>MSTYEGRWKTVKVEIEDGIAFVILNRPEKRNAMSPTLNREMIDVLETLEQDPAAGVLVLTGAGEAWTAGMDLKEYFREVDAGPEILQEKIRREASQWQWKLLRMYAKPTIAMVNGWCFGGGFSPLVACDLAICADEATFGLSEINWGIPPGNLVSKAMADTVGHRQSLYYIMTGKTFGGQKAAEMGLVNESVPLAQLREVTIELARNLLEKNPVVLRAAKHGFKRCRELTWEQNEDYLYAKLDQSRLLDTEGGREQGMKQFLDDKSIKPGLQAYKR[4x];> MSTYEGRWKTVKVEIEDGIAFVILNRPEKRNAMSPTLNREMIDVLETLEQDPAAGVLVLTGAGEAWTAGMDLKEYFREVDAGPEILQEKIRREASQWQWKLLRMYAKPTIAMVNGWCFGGGFSPLVACDLAICADEATFGLSEINYGIPPGNLVSKAMADTVGHRQSLYYIMTGKTFGGQKAAEMGLVNESVPLAQLREVTIELARNLLEKNPVVLRAAKHGFKRCRELTWEQNEDYLYAKLDQSRLLDTEGGREQGMKQFLDDKSIKPGLQAYKR;> MSTYEGRWKTVK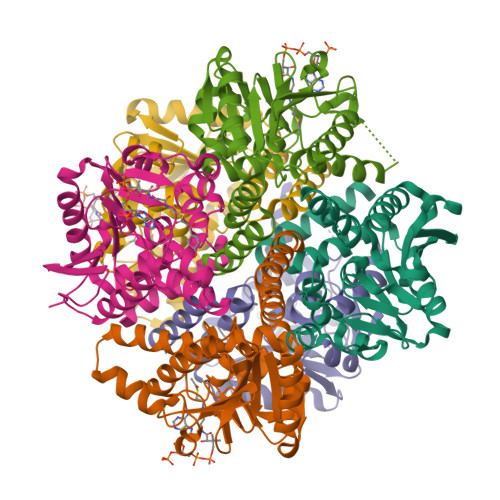VEIEDGIAFVILNRPERRNAMSPTLNREMIDVLETLEQDPAAGVLVLTGAGEAWTAGMDLKEYFREVDAGPEILQEKIRREASQWQWKLLRMYAKPTIAMVNGWCFGGGFSPLVACDLAICADEATFGLSEINWGIPPGNLVSKAMADTVGHRQSLYYIMTGKTFGGQKAAEMGLVNESVPLAQLREVTIELARNLLEKNPVVLRAAKHGFKRCRELTWEQNEDYLYAKLDQSRLLDTEGGREQGMKQFLDDKSIKPGLQAYKR>SGHHEDSTDEPSESSEPCCDSCVCTKSIPPQ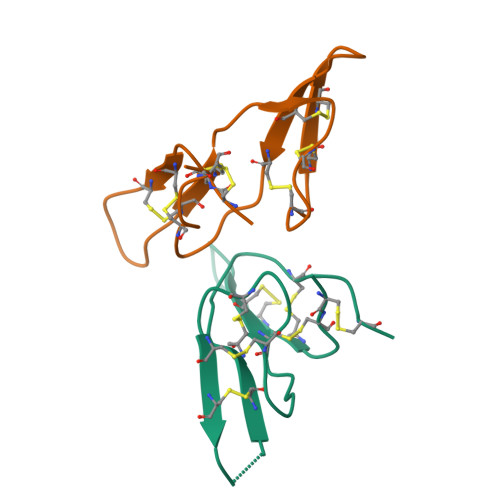CHCTNIRLNSCHSGCKSCLCTFSIPGSCRCLDIANFCYKPCKS[2x]>[2x]LK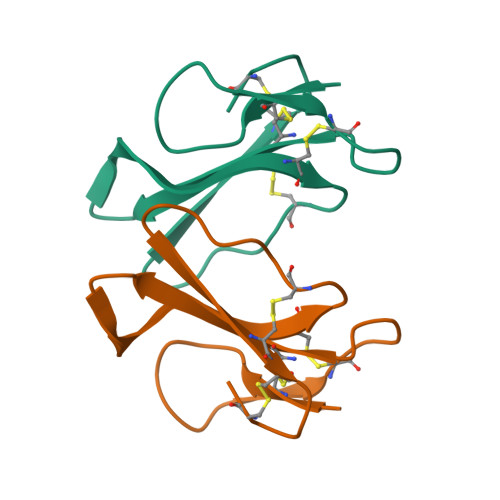CHNKLVPFLSKTCPEGKNLCYKMTLMKMPKIPIKRGCTDACPKSSLLVKVVCCNKDKCN>GSGLNIKENDLPGIGKKFEIETRSHEKMTIIIHDDGR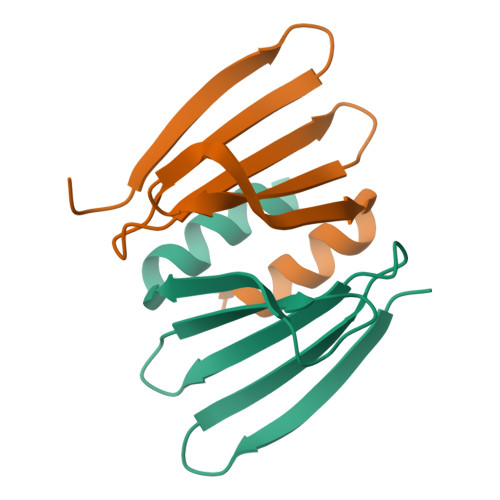REIYRFNDRDPDELLSNISLDDSEARQIAAILGG[2x]>[2x]MGSSHHHHHHSSGLVPRGSHMASMEST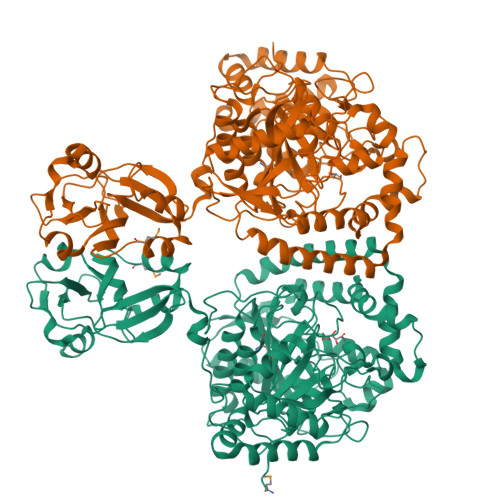LGWSVQDWLSFHSKSTPTKSLELLENLLKSQKPAPEDPAWISLIPVEDLHHQWNILQSKSNKEELPLYGVPIAVKDNIDYKGLPTTAACPSYLYQPTRDSYVVELLRDAGAVVIGKTNLDQFATGLVGTRSPYGKTPCVFNDKYVSGGSSAGSASVVGRGIVPLSLGTDTAGSGRVPAALNNLIGLKPTKGAFSCRGVVPACKSLDCVSVFALNLSDAEIAFKVMNKPDLLEDEYSREFPKNPISQYPKDLTIAIPKEVPWFGETENPKLYTKAVASLKNTGAKIVVVDFEPLLELARCLYEGAWVAERYCATRDFLATNPPESSLDETVVNIIKGAVKFDAADAFKFEYKRQGILQKVNLLLKDIDVLCVPTCPLNPKLEEVAQEPVLVNSRQGTWTNFVNLADLAALAVPSGFRSDGLPNGITLIGKKFSDYALLDLAKRFFSVAFPNNSRTYGKFVDRRITVEDELDGPSKDTLNGVKLAVVGAHLKGLPLHWQLQKCNATYLSSPKTSNNYKLYALPKVGPVLKPGLRRVNDGTGSQIQLEVYSVPYDRFGDFIAMVPEPLGIGSVELESGEWVKSFICEEFGYTQQGTVDITKFGGFKPYIEHIQVTEAQKK> MGLNFFRKAAPEVRTEPVAERKASVTGRIVAMASGAGRPVWGPRDTVSLMRTGFAGNPVGFRSVKLIAEATAAVPLICQDAERRYEIHPVLDLLRRPNAGQGRAELFEALIGQILLSGNGYLEAVCPEPGVPRELHVLRSDRMAVVPGADGWPVGYDYTVGGRKHRFDMTGHPDPICHIKSFHPTDDHYGLSPMQAAAVALDVHNAASAWSKALLDNAARPSGAIIYKGADGQGVLAPEQYERLIFEMETHHQGARNAGRPMLLEGGLDWKPMGFSPSDMEFHETKAAAAREIALAFGVPPMLIGIPGDATYANYAEANRAFYRLTV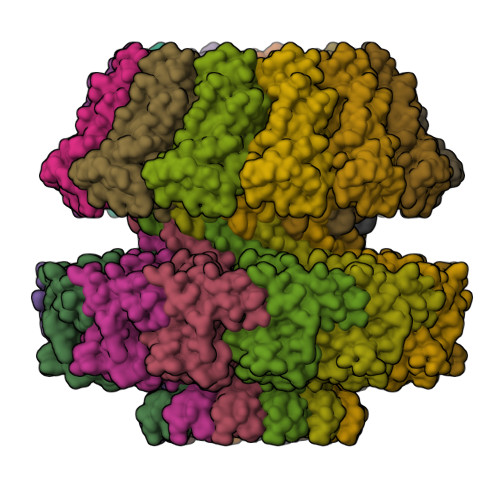LPLLTRVSAALAWWLSGYLGAQIELKPDLDQVPALAVERDQLWARIGAAGFLSNSEKRVLLGLPPT;> MMLNEVTAVPGTALPVAEFRDHLRLGTGFADLGAEDAALLSYLRAAIAAIEGRTAKALISRGFRLALTAWRWGDMQTLPIAPVATVTALRLVDAAGVETPVAAGWRLVPDMARPRIEALGAMLPMIPTGGRVEIDFTAGFGASWSALPVDLAQAVFLLAAQYYELRHDGAAEGGAMPFGVMALIERWRTVRVLGGRP>[2x]MQANDGHWYLFTADGTAASRVAKWAGTYYYFDPQTHLRVDDNYVQSQWGDWYMFGKDGRIATGLYKWDKNNQWYYFDPVTYLKVTNKWVDGNYYDEDGAQAISKLVTINNRLYYFDDQGKEISNQFRTIHGDKYYFGNDSAAVTGQQTIDGKVYKFSNYGYLLGNRYGKIENGKLNIYSLADNSLIKTVEAGPWENMAYSMDSNSINNIDGYISYTGWYRPYGTSQDGKTWYPTTVADWRPILMYVWPSKDVQVKFIQYFVNHGYENSNYGLTAGSVKDLSENTASIKLNEVAQNLRYVIEQHVVAAKSTSQLANDINNFITTIPELSKASELSVVNSYGYKPDNSGSVDDDQVIFVNNDSKNQKIGNTSYADSNYRLMNRTINNQNGDNNSDDSPELLVGNDIDNSNPVVQAENLNWEYFLLNYGKFMNYNPNGNFDG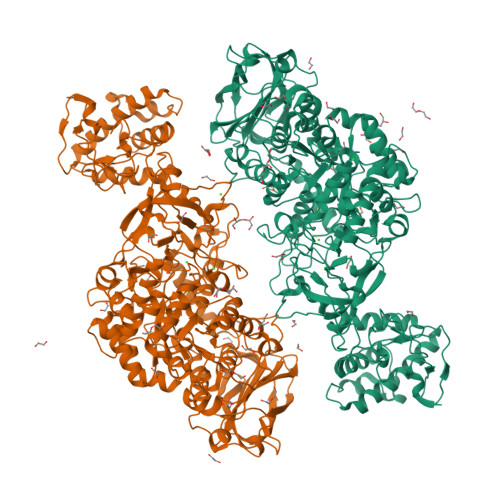FRIDAADNIDADVLDQAAQLINSIYNTKGNQANANDHLIYNEGYHLGAANMLDRKSNPELYMDSGYFYTLENVLGRASDRDDINNLITNSIVNRQNDVSENVATPNWSFVTNHDQRKNLINQIVIDDHPGVADIMSDGYKAEYVNQAWKEFYADQARTDKKYTQYNLPAQYALLLTNKDTVPQVYYGDLYDETDQYMQNKSVYYDAITTLMKARKSYVSGGQSMIKINDHLLTSVRYGKGIIDGNVSMTDILGRNSGIAVVVGNDAQMANQTISINMGKAHANQAYKQLLGTIDSGLTSSDTTIYHTDSNGVLNVTVKGYSNPYVSGYLGVWVPLNGGANITTKASEVTNQSDKTYSSNAALDSHVIYEDFSLFQPEPTSKAEHAYNIIADNASLFNELGITDFWMAPAYTPFNTSRYNEGYSMTDRYNLGTEANLTKYGSGEELSNAIAALHDAGLKVQEDLVMNQMIGFSGQEAVTVTRTDGHAKQLTVDGKTFANQIYFAYTRGGGEGQKNYGGKYLDELQKKYPELFTTKAVSTGVAPDPSVHITEWSAKYQNGTSLQNIGIGLAVKLANGDYAYLNDSNNKAFNTTLPETMSSADYYANIEDD2-(2-chloro-4-nitrophenoxy)-5-ethyl-4-fluorophenol | C14 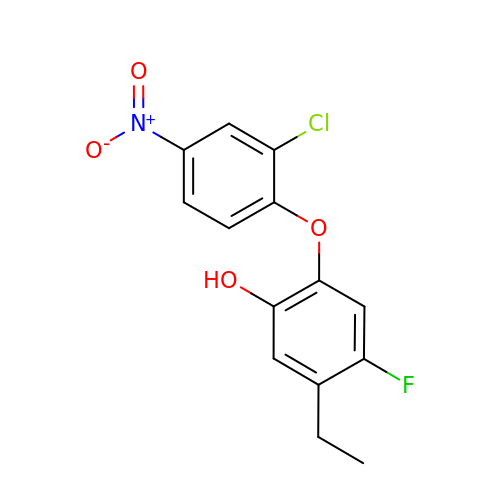H11 Cl F N O4 | RGNGXGXBSAFDJR-UHFFFAOYSA-N> MQNNNEFKIGNRSVGYNHEPLIICEIGINHEGSLKTAFEMVDAAYNAGAEVVKHQTHIVEDEMSDEAKQVIPGNADVSIYEIMERCALNEEDEIKLKEYVESKGMIFISTLFSRAAALRLQRMDIPAYKIGSGECNNYPLIKLVASFGKPIILSTGMNSIESIKKSVEIIREAGVPYALLHCTNIYPTPYEDVRLGGMNDLSEAFPDAIIGLSDHTLDNYACLGAVALGGSILERHFTDR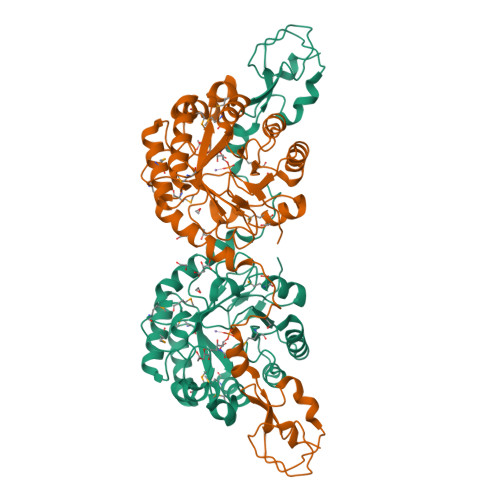MDRPGPDIVCSMNPDTFKELKQGAHALKLARGGKKDTIIAGEKPTKDFAFASVVADKDIKKGELLSGDNLWVKRPGNGDFSVNEYETLFGKVAACNIRKGAQIKKTDIE>[2x]DFFRDEAERIMRDSPVIDGHNDLPWQLLDMFNNRLQDERANLTTLAGTHTNIPKLRAGFVGGQFWSVYTPCDTQNKDAVRRTLEQ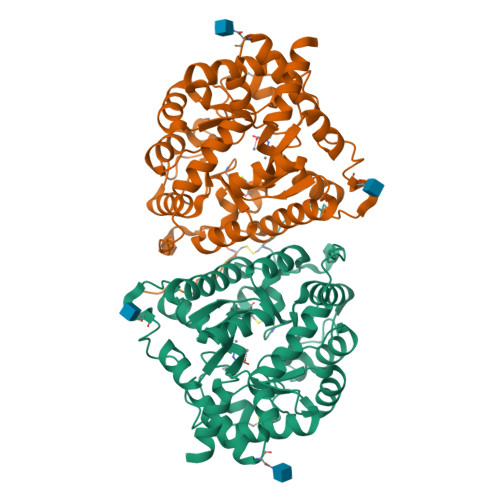MDVVHRMCRMYPETFLYVTSSAGIRQAFREGKVASLIGVEGGHSIDSSLGVLRALYQLGMRYLTLTHSCNTPWADNWLVDTGDSEPQSQGLSPFGQRVVKELNRLGVLIDLAHVSVATMKATLQLSRAPVIFSHSSAYSVCASRRNVPDDVLRLVKQTDSLVMVNFYNNYISCTNKANLSQVADHLDHIKEVAGARAVGFGGDFDGVPRVPEGLEDVSKYPDLIAELLRRNWTEAEVKGALADNLLRVFEAVEQASNLTQAPEEEPIPLDQLGGSCRTHYGYSS3-[3,4-bis(fluoranyl)phenyl]-1,4,6,7-tetrahydroimidazo[2,1-c][1,2,4]triazine | C11 H10 F2 N4 | 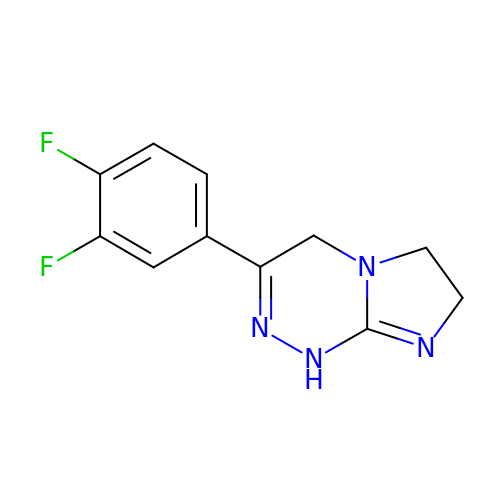HQCSFWFWWSDEFP-UHFFFAOYSA-N> MAAAAWLQVLPVILLLLGAHPSPLSFFSAGPATVAAADRSKWHIPIPSGKNYFSFGKILFRNTTIFLKFDGEPCDLSLNITWYLKSADCYNEIYNFKAEEVELYLEKLKEKRGLSGKYQTSSKLFQNCSELFKTQTFSGDFMHRLPLLGEKQEA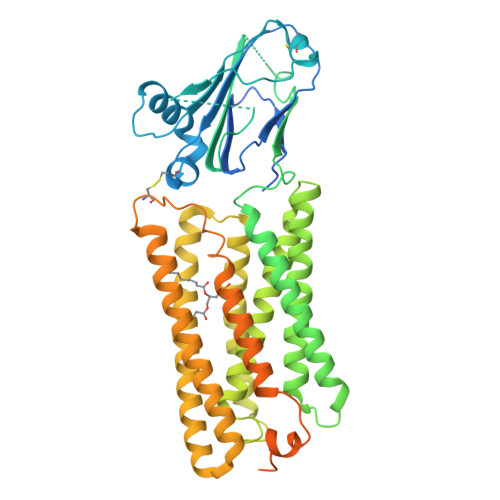KENGTNLTFIGDKTAMHEPLQTWQDAPYIFIVHIGISSSKESSKENSLSNLFTMTVEVKGPYEYLTLEDYPLMIFFMVMCIVYVLFGVLWLAWSACYWRDLLRIQFWIGAVIFLGMLEKAVFYAEFQNIRYKGESVQGALILAELLSAVKRSLARTLVIIVSLGYGIVKPRLGVTLHKVVVAGALYLLFSGMEGVLRVTGAQTDLASLAFIPLAFLDTALCWWIFISLTQTMKLLKLRRNIVKLSLYRHFTNTLILAVAASIVFIIWTTMKFRIVTCQSDWRELWVDDAIWRLLFSMILFVIMVLWRPSANNQRFAFSPLSEEEEEDEQKEPMLKESFEGMKMRSTKQEPNGNSKVNKAQEDDLKWVEENVPSSVTDVALPALLDSDEERMITHFERSKMESNSLEVLFQ(2Z)-4-[3-(decyloxy)phenyl]-2-hydroxy-4-oxobut-2-enoic acid 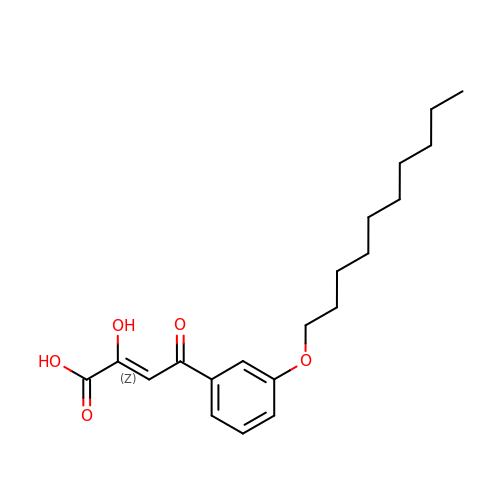| C20 H28 O5 | QHFZPXDAWCLNPO-CYVLTUHYSA-N> MNSITHAEFEFSLLENVKYETEDEVPIVLEYKEEIINLIKKFSNSGQSGMSAPITASIITNCIKNLMAFKPIGPLVGNEEEWNYNSDDSFQNNRLSAVFKTGLNGKPYYLDAITFVGEEEYDTFHGHVEGISSRQYLKGFPFFPKTFYINVY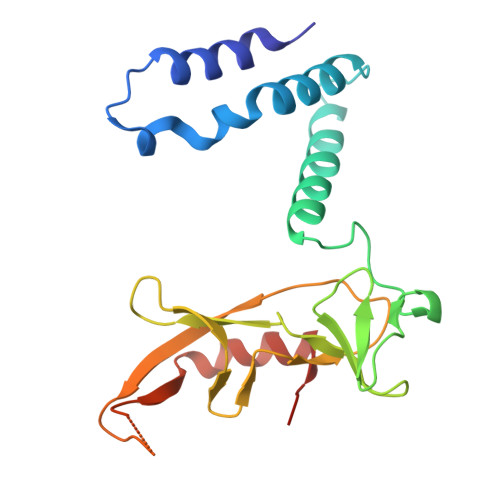KDFENKDENNLCSGDDGEYTYRIKYPEQLEEVFNYYDKFTKE> MSMLGERRRGLTDPEMA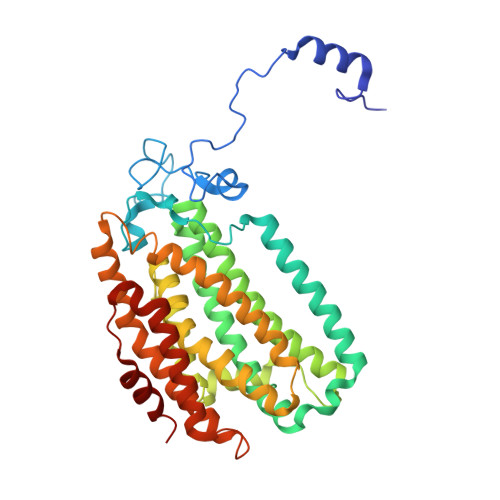AVILKALPEAPLDGNNKMGYFVTPRWKRLTEYEALTVYAQPNADWIAGGLDWGDWTQKFHGGRPSWGNETTELRTVDWFKHRDPLRRWHAPYVKDKAEEWRYTDRFLQGYSADGQIRAMNPTWRDEFINRYWGAFLFNEYGLFNAHSQGAREALSDVTRVSLAFWGFDKIDIAQMIQLERGFLAKIVPGFDESTAVPKAEWTNGEVYKSARLAVEGLWQEVFDWNESAFSVHAVYDALFGQFVRREFFQRLAPRFGDNLTPFFINQAQTYFQIAKQGVQDLYYNCLGDDPEFSDYNRTVMRNWTGKWLEPTIAALRDFMGLFAKLPAGTTDKEEITASLYRVVDDWIEDYASRIDFKADRDQIVKAVLAGLK>MEHDERTHVPVELRAAGVVLLNERGDILLVQEKGIPGHPEKA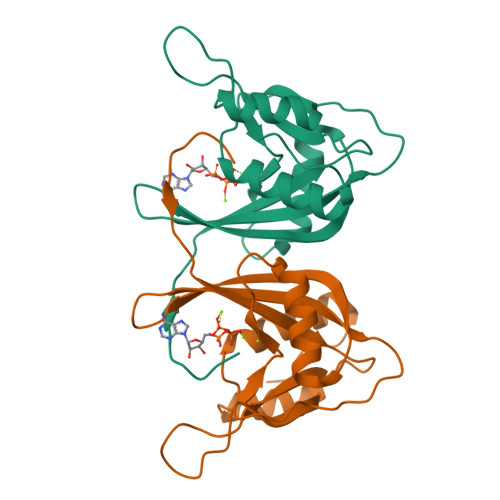GLWHIPSGAVEDGENPQDAAVREACEETGLRVRPVKFLGAYLGRFPDGVLILRHVWLAEPEPGQTLAPAFTDEIAEASFVSREDFAQLYAAGQIRMYQTKLFYADALREKGFPALPV[2x]>[4x]MLLQASQATQSVWKTLNKWLPPLSRDKDWWWKTLGPQINTLLTEADYDLNERYEALLLLYRWVVPEMGPRPRSSVAPSKSFMTDDHSPIEYSWKWISGNKKPEIRYAVELVSPLAGSKQDPFNQIPTRNLVYNLAKIIPELDLTWFEHFWHELLGPGSPTTSTSGVLTKGSTVFAALEMLHGHLSVKVYFIPVETPDFSAWHQIKHAIEASGCPNLEALNHVDAYLSSHDDGRQLRPFMLAI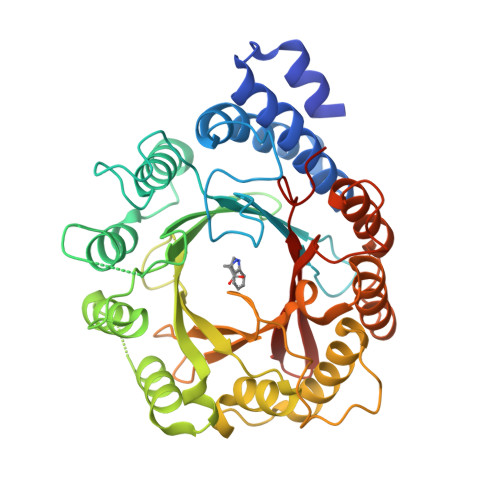DLVEPAASRLKIYARSNQTSFRFVRDVMTIGGLRTDLDRSIEKFSDLWKRALGLDPDTPPEDELPKVDHLTSGAVFNFDVAPKSQIPEVKAYIPVRHYANNDLQAALGLIGYLEDHGHGGYSQSYLRGLDMLAPSGQLDQATGVQTYFAVACQGEDLSLTSYLNPQFYAAFQEPERT>GPSGTSHMLTLARQQQRQNIRWLLSLSVLMLLALLLSLSAGEQWISPGDWFTPRGELFVWQIRLPRTLAVLLVGAALAISGAVMQALFENPLAEPGLLGVSNGAGVGLIAAVLLGQGQLPNWALGLSAIAGALIITLILLRFARRHLSTSRLLLAGVALGIISSALMTWAIYFSTSVDLRQLMYWMMGGFGGVDWRQSWLMLALIPVLLWISSQSRPMNMLALGEISARQLGLPLWFWRNVLVAATGWMVGVSVALAGAIGFIGLVIPHILRLSGLTDHRVLLPGCALAGASALLLADIVARLALAA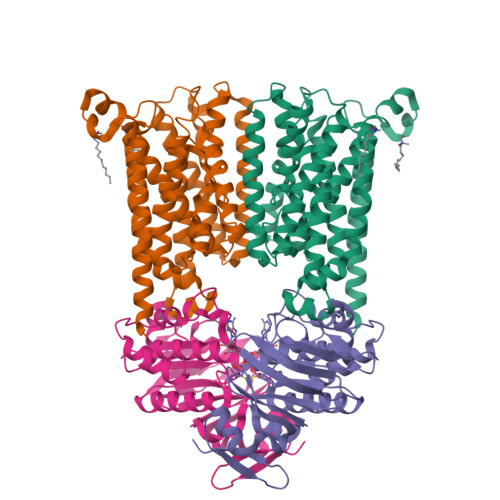AELPIGVVTATLGAPVFIWLLLKAGR[2x];>MSIVMQLQDVAESTRLGPLSGEVRAGEILHLVGPNGAGKSTLLARMAGMTSGKGSIQFAGQPLEAWSATKLALHRAYLSQQQTPPFATPVWHYLTLHQHDKTRTELLNDVAGALALDDKLGRSTNQLSGGEWQRVRLAAVVLQITPQANPAGQLLLLDQPMCSLDVAQQSALDKILSALSQQGLAIVMSSHDLNHTLRHAHRAWLLKGGKMLASGRREEVLTPPNLAQAYGMNFRRLDIEGHRMLISTI[2x]>MRLDGKTALITGSARGIGRAFAEAYVREGARVAIADINLEAARATAAEIG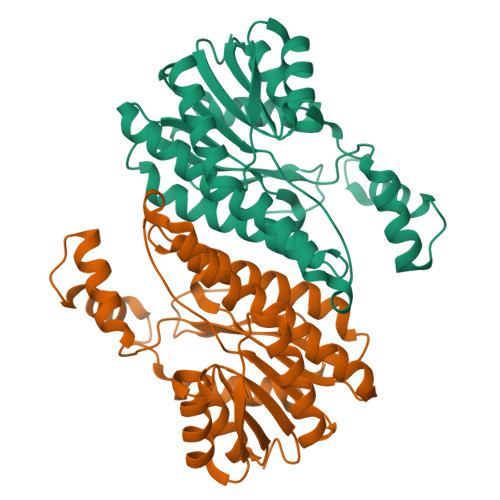PAACAIALDVTDQASIDRCVAELLDRWGSIDILVNNAALFDLAPIVEITRESYDRLFAINVSGTLFMMQAVARAMIAGGRGGKIINMASQAGRRGEALVGVYCATKAAVISLTQSAGLNLIRHGINVNAIAPGVVDGEHWDGVDAKFADYENLPRGEKKRQVGAAVPFGRMGRAEDLTGMAIFLATPEADYIVAQTYNVDGGNWMS[2x]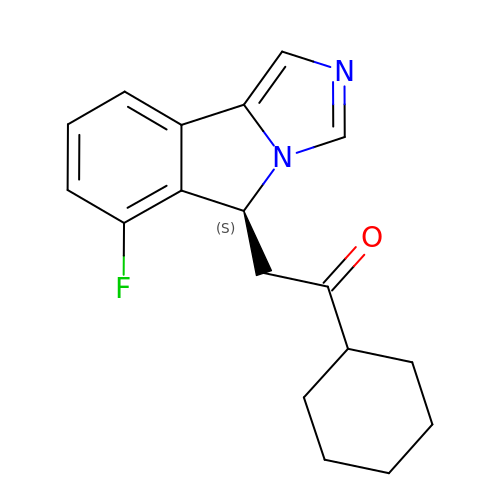1-cyclohexyl-2-[(5~{S})-6-fluoranyl-5~{H}-imidazo[1,5-b]isoindol-5-yl]ethanone | C18 H19 F N2 O | IDAMUBBXWPKKDM-HNNXBMFYSA-N The cap intermediate is methylated by the RNA guanine N-7 methyltransferase, utilising the methyl donor, AdoMet, to create the mature cap, m7GpppN, and byproduct, AdoHcy (S-adenosyl homocysteine). In mammals, RNA guanylyltransferase and 5′-triphosphatase (RNGTT/CE) caps the nascent transcript and RNA guanine-7 methyltransferase (RNMT) methylates the cap. Human RNMT is a 476 amino acid nuclear protein consisting of a catalytic domain (residues 121–476), with homology to other eukaryotic cap methyltransferases and an N-terminal regulatory domain (residues 1–120), that mediates recruitment to transcription initiation sites. RNMT also has an activating subunit, RAM (RNMT-activating miniprotein).

In order to characterise RNMT lobe function, a deletion mutant was engineered in which lobe residues 416–456 are replaced with a GSGG linker (RNMTΔ416–456). Despite the absence of the lobe in this mutant and in thermolysin-cleaved RNMT, the crystal structures are not altered significantly compared to RNMT–RAM (RMSD 0.5 Å). Moreover, no substantial differences in the position of key active site residues were observed in the crystals upon deletion of the lobe. Removal of the lobe significantly reduced cap methyltransferase activity, over a titration of RNMT, with or without equimolar RAM 2–45, indicating that the lobe has a significant role in catalysis. Since RAM can partially activate RNMTΔ416–456, it activates by mechanisms additional to stabilising the lobe (discussed later). Many lobe residues interact with RAM and deletion of the lobe considerably weakened the RNMT-RAM interaction to below the limit of detection in GST-pulldown. Deletion of the lobe did not impact on SAMFP binding to the RNMT monomer, however RAM 2–45 was unable to stimulate SAMFP binding to RNMTΔ416–456, consistent with a defect in RAM binding. Removal of the lobe in RNMTΔ416–456 leads to a significant increase in flexibility of both the α-helix hinge and helix A in simulations. In agreement, the average isotropic B factor values for the α-helix hinge compared to the whole protein within the same crystal structure displays a marked increase on lobe removal (average B factor hinge = 28.2 Å2 versus main chain = 23 Å2), in comparison to the RNMT-RAM complex (average B factor hinge = 24.4 Å2 versus main chain = 24.4 Å2). In summary, deletion of the lobe reduces the catalytic activity of RNMT and impairs its ability to bind and be activated by RAM.

>SRIFYLRNFNNWMKSVLIGEFLEKVRQKKKRDITVLDLGCGKGGDLLKWKKGRINKLVCTDIADVSVKQCQQRYEDMKNRRDSEYIFSAEFITADSSKELLIDKFRDPQMCFDICSCQFVCHYSFESYEQADMMLRNACERLSPGGYFIGTTPNSFELIRRLEASETESFGNEIYTVKFQKKGDYPLFGCKYDFNLEGVVDVPEFLVYFPLLNEMAKKYNMKLVYKKTFLEFYEEKIKNNENKMLLKRMQGGSGSKSEWEATSIYLVFAFEKQQ[2x]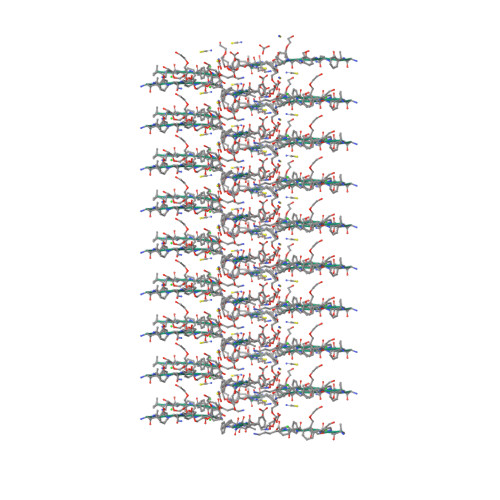> LFKFFK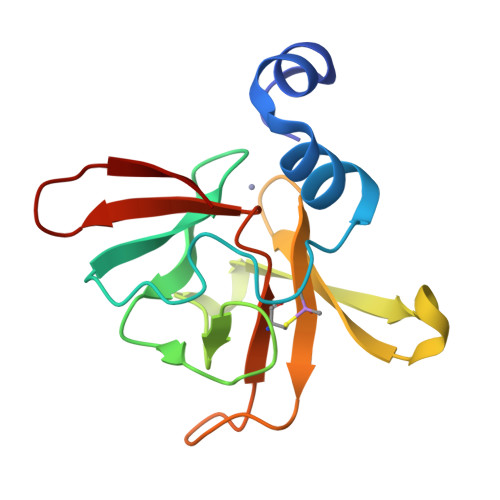>[2x]MANKPSAEELKKNLSEMQFYVTQNHGTEPPFTGRLLHNKRDGVYHCLICDAPLFHSQTKYDSGCGWPSFYEPVSEESIRYIKDLSHGMQRIEIRCGNCDAHLGHVFPDGPQPTGERYCVNSASLRFTDGENGEEING> GKRQWALEDFEIGRPLGKGKFG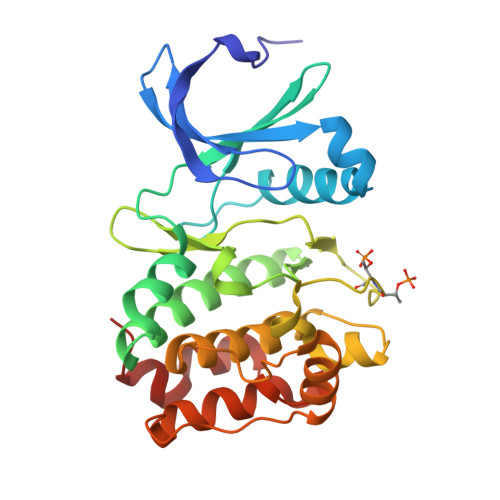NVYLAREKQSKFILALKVLFKAQLEKAGVEHQLRREVEIQSHLRHPNILRLYGYFHDATRVYLILEYAPLGTVYRELQKLSKFDEQRTATYITELANALSYCHSKRVIHRDIKPENLLLGSAGELKIADFGWSVHAPSSRRTTLCGTLDYLPPEMIEGRMHDEKVDLWSLGVLCYEFLVGKPPFEANTYQETYKRISRVEFTFPDFVTEGARDLISRLLKHNPSQRPMLREVLEHPWITANSSKPS> SQSTRKKSR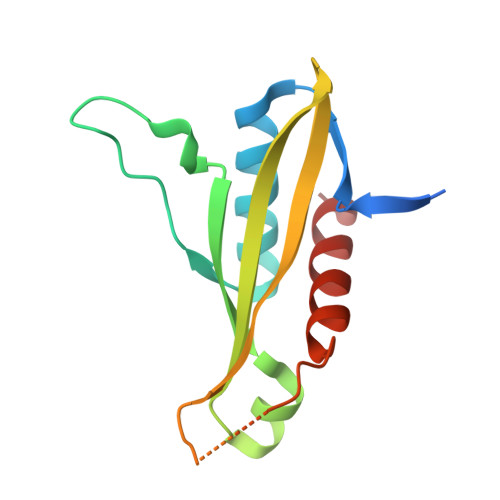RNKWHFGVRCRGDAPEILLAVYRALQRAGAQFTVPKPVNGKYRSDMYTIKSRWEIPHCKREGKNTYAYIELQLYEVMPGCFMLDVKSNGYKDIYSHPERTADHGMDDLKSSFPFLDLCAMLVCKLFSA> GPGSMSDTEYLARAEAVLAAVERTVDVANDGDHDIDLERNGSVLTLTFENGSKIIVNLQPPMKEVWIAAKAGGFHYRFIDGEWRDTRTGTE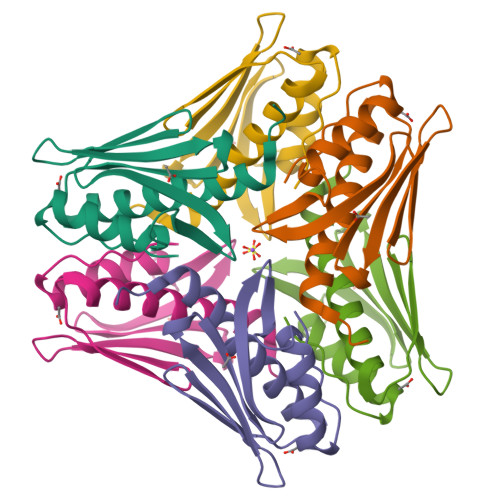FFSALTDYATQQAGLPITFSA> XLPLYTSPSLPNITLGL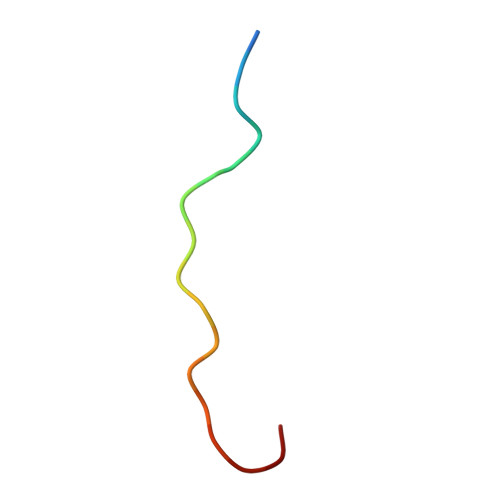P Compared to TbREX1, TbREX2 and TbDSS-1, TbRND is unique, as it belongs to the RNase D (RND) group within the DEDD exoribonuclease superfamily. Like E. coli RNase D (EcRND), Saccharomyces cerevisiae Rrp6 (ScRrp6), and all other RND family proteins, TbRND possesses a single 3′-5′ exoribonuclease (Exo) domain. EcRND and ScRrp6 possess an HRDC (helicase and RNase D C-terminal) domain at the C-termini whereas TbRND contains a predicted CCHC zinc-finger domain (ZFD) at its C-terminus. Depletion of TbRND results in extended gRNA tails in vivo, whereas, overexpression of TbRND leads to a substantial reduction in the total gRNA population and the subsequent inhibition of mRNA editing.

Although no crystals grew for the mixture of RNA and RND-WT, we successfully solved the structure for a complex of RNA-12U bound to the TbRND ΔZF_3–4 mutant (amino acids 41–341), a truncation in which ZF3 and ZF4 were deleted. The structure was termed ΔZF_3–4/RNA-12U and refined to high resolution (1.77 Å). Of the 12 nucleotides in RNA-12U, 10 were well-ordered and labeled R0 to R9 from the 3′ end. The Zinc fingers, ZF1 and ZF2, of TbRND mainly interact with the nucleotides at the R5–R9 region. Although RND-Exo alone does not show clear RNA1-binding affinity in vitro, the Exo domain forms extensive interactions with the RNA in the ΔZF_3–4/RNA-12U complex structure, mainly recognizing nucleotides R0-R4 located at the 3′-end of RNA-12U. The crystals of the ΔZF_3–4/RNA-12U complex were grown in the presence of 10 mM CaCl2. In the structure, two well-defined Ca2+ ions were captured in the active site in a hexacoordinated octahedral-like geometry. The A-site ion is coordinated by the side chains of the Asp80, Glu82, and Asp230 residues, as well as the OP1 atom of R0 and two water molecules. The B-site ion is coordinated by the side chain of Asp80, the OP1 atom of R0, and three water molecules. Several structures were determined, including a ΔZF_3–4/RNA-12U complex, which represents the first ternary structure composed of native RND protein, substrate RNA, and coordinating cations.

> TSSATSSSSMILKYPYRVVDTHEKLKEAVTSLQGARSIALDIEAFCTTDQAKQLGRISLVQACSDAKPVVFLFDVLTLTPDVFVKDMQSLLSDREIRKLFFDCRRDVEALSCQLGVKPEGVLDLQVFFTAIQWKLRSVNRRSGMGYVLKSVAGLTRQEGDSAVQTAMTLGNRPVWDIRPLPDHFLEYAAGDVRHILLLSNYLVGNKDVPVDVVAVERLTAQYVEHYAVGKPVITEADATPAEVNRAWLERYIGPGGGCHFCGAKGHTEAECFKKQNGKAKCSFCGEVGHTARNCFKKHPQLL> MAEQEDIILEKPEDGLNQPRLDESLEGFKGQEGQAPEDEEFASLPEELPQENSESGFKFTRESAPEDVSTFEEVESQEPTPWYKDRKFMSLVGLSLGIICILVFTLFYLTFSEGKIKPDIIASKPLEQPVVMPDESYKYNDMQRIDGMIQKANALYLKGEVEQALKVYEQVAVYNESLSNYNLGVSQMNENKFQEAFESFKKAIANGENQSVAAINAAVCALKLNDKEKFRYYIDLAQVYLPKEGKSKLYDYYLSLINYYKGYYPEALQMLQRTDMEPYSDVAKYLSAKIYAKMDFDSKAIQQLNSQGNFESSLSLG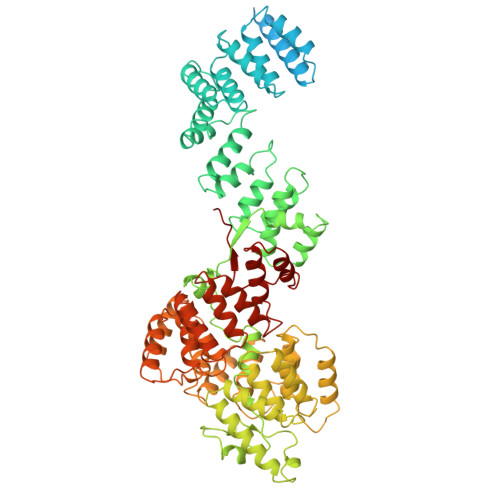LLYARIGEYAKAKVALSTAMKIERDFNQSLAALTLVDIKTGNYQDMLARLQNSYDNDKDRYKILDAYKIQVRLNKDLFNIAVAQNSFSKDLLKKQKDQFDLLFYFAPYQVFDSKQAALYIKKANVTDFVDDSADAGVYLNTSKALSSTNVKIANIINYALNQKLRLANQEFQKLIKDYPEHSILHYNLALTYAQMQNYELAYKHFSSSYHLNPKNYLAGAFAMFCAKLIDIDTTKLYNEILDNIAADSNFKANMQKSMLFLVNNNYISMLPYLDETKKDTPLSLIFEAIVAKNNNLNNQVDVKIAKLRSELPEDILANILYFNSLNSNLNIKEYAQNAQIHFKNLKLDYRSVFGGPNIAREFYVNLMHIAGLLNLERQKIKELINVSGAKDEGILQTLAYLDIFAQQYEEAYALYNSLIDDYGAKDTKTLFLAAVAAIGANNPNSAIALLQLSKLTDKNNKESKAALGMLYQEVKNYEAAISQYKTLPNNFKSEFFTFDINNN> MKKLIPILEKIPEVELPVKEITFKE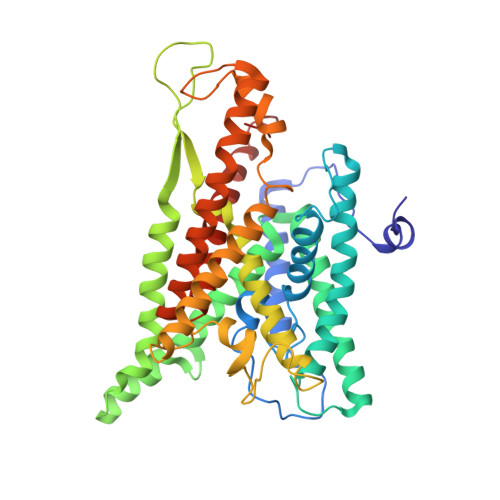KLKWTGIVLVLYFIMGCIDVYTAGAQIPAIFEFWQTITASRIGTLITLGIGPIVTAGIIMQLLVGSGIIQMDLSIPENRALFQGCQKLLSIIMCFVEAVLFVGAGAFGILTPLLAFLVIIQIAFGSIILIYLDEIVSKYGIGSGIGLFIAAGVSQTIFVGALGPEGYLWKFLNSLIQGVPNIEYIAPIIGTIIVFLMVVYAECMRVEIPLAHGRIKGAVGKYPIKFVYVSNIPVILAAALFANIQLWGLALYRMGIPILGHYEGGRAVDGIAYYLSTPYGLSSVISDPIHAIVYMIAMIITCVMFGIFWVETTGLDPKSMAKRIGSLGMAIKGFRKSEKAIEHRLKRYIPPLTVMSSAFVGFLATIANFIGALGGGTGVLLTVSIVYRMYEQLLREKVSELHPAIAKLLNK> PKNKARRRT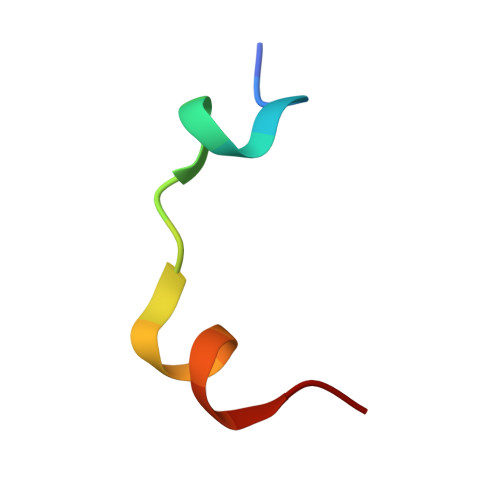TTQMELLYAD> MDPFASTRTFNLAMTDIGEMYFMPPLMEALAQRAPHIQISTLRPNAGNLKEDMESGAVDLALGLLPELQTGFFQRRLFRHRYVCMFRKDHPSAKSPMSLKQFTELEHVGVVALNTGHGEVDGLLERAGIKRRMRLVVPHFIAIGPILHSTDLIATVPQRFAVRC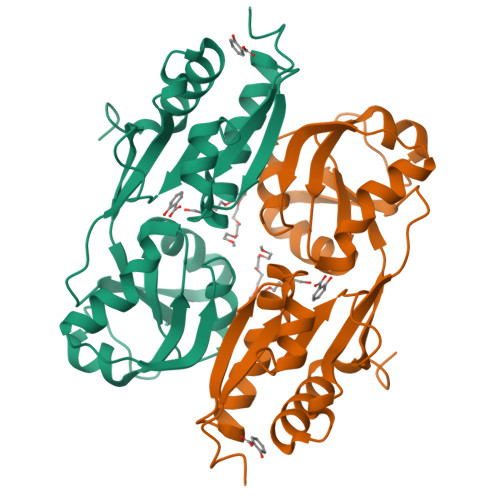EVPFGLTTSPHPAKLPDIAINLFWHAKYNRDPGNMWLRQLFVELFSEAHHHHHH Here, we identify an evolutionarily conserved hexapeptide sequence as the major aggregation-prone region (APR) of gastrointestinal peptides of the glucagon family: xFxxWL. We determine nine polymorphic crystal structures of the APR segments of glucagon-like peptides 1 and 2, and exendin and its derivatives. We propose that the pH-dependent changes of the protonation states of glutamate/aspartate residues of APRs initiate switching between the amyloid and the folded, monomeric forms of the hormones. Our results highlight the dual role of short aggregation core motifs in reversible amyloid formation and receptor binding.

Four polymorphic crystal forms were grown from solutions of APRTc5b. Interaction networks formed in crystals of polymorphs A and C are essentially identical. Aromatic side chains form a cluster in which acetonitrile or ethanol is also present, while TFA forms multiple H-bonds with termini and Trp side chains. As the concentration of EtOH was reduced from 30% to 10% in the crystallization solution (keeping all the other parameters identical), the entire cross-β scaffold rearranged from parallel to antiparallel relative orientation. On the other hand, nearly identical polymorphic structures were obtained from the crystals grown in 10% EtOH and 30% ACN (polymorph A vs. C). The two different organic solvent molecules are located approximately at the same place within the crystal, despite their different structures and chemical properties. In polymorphs A and C of APRTc5b, an acetonitrile/ethanol solvent molecule is incorporated in the aromatic cluster, leading to somewhat larger ring-to-ring distances as compared to those of APRex-4. In the presence of organic solvents, the exendin-like structures adopted more compact crystal forms, in which opposing side chains of the steric zippers interact with each other.

>[2x]LYIQWL> TDRYTIHSQLEHLQSKYIGTGHADT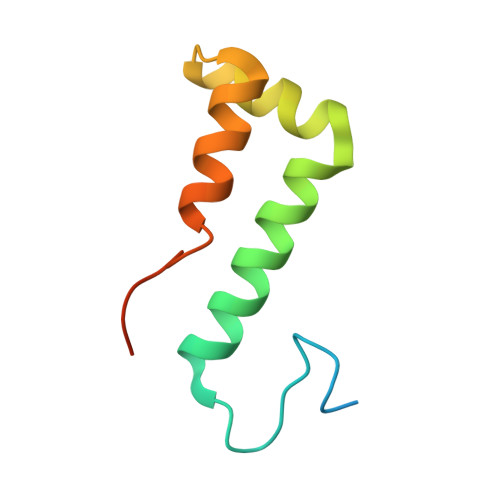TKWEWLVNQHRDSYCSYMGHFDLLNYFAIAENESKARVRFNLMEKMLQPCGPPADKPEEN> MEDPLIGRDSLGGGGTDRVRRSEAITHGTPFQKAAALVDLAEDGIGLPVEILDQSSFGESARYYFIFTRLDLIWSLNYFALLFLNFFEQPLWCEKNPKPSCKDRDYYYLGELPYLTNAESIIYEVITLAILLVHTFFPISYEGSRIFWTSRLNLVKVACVVILFVDVLVDFLYLSPLAFDFLPFRIAPYVRVIIFILSIRELRDTLVLLSGMLGTYLNILALWMLFLLFASWIAFVMFEDTQQGLTVFTSYGATLYQMFILFTTANNPDVWIPAYKSSRWSSVFFVLYVLIGVYFVTNLILAVVYDSFKEQLAKQVSGMDQMKRRMLEKAFGLIDSDKNGEIDKNQCIKLFEQLTNYRTLPKISKEEFGLIFDELDDTRDFKINKDEFADLCQAIALRFQKEEVPSLFEHFPQIYHSALSQQLRAFVRSPNFGYAISFILIINFIAVVVETTLDIEESSAQKPWQVAEFVFGWIYVLEMALKIYTYGFENYWREGANRFDFLVTWVIVIGE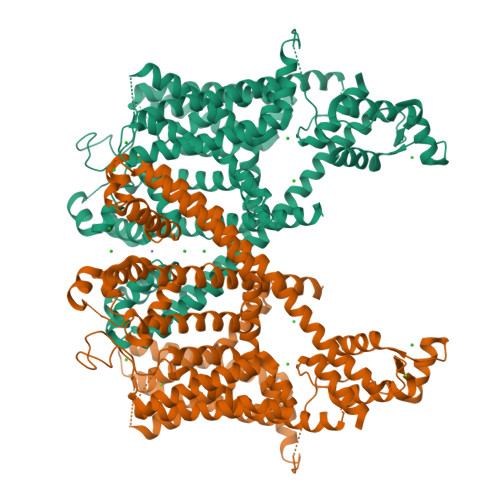TATFITPDENTFFSNGEWIRYLLLARMLRLIRLLMNVQRYRAFIATFITLIPSLMPYLGTIFCVLCIYCSIGVQVFGGLVNAGNKKLFETELAEDDYLLFNFNDYPNGMVTLFNLLVVNNWQVWMESYKDLTGTWWSITYFVSFYVITILLLLNLVVAFVLEAFFTELDLEEEEKCQGQDSQEKRNRRRSAGSKSRSQRVDTLLHHMLGDELSKPECSTSDTSTAGLV> MSKLTQVFKQTKLCIGYLTAGDGGTSYTIEAAKALIQGGVDILELGFPFSDPVADNPEIQVSHDRALAENLTSETLLEIVEGIRAFNQEVPLILYSYYNPLLQRDLDYLRRLKDAGINGVCVIDLPAPLSHGEKSPFFEDLLAVGLDPILLISAGTTPERMSLIQEYARGFLYYIPCQATRDSEVGIKEEFRKVREHFDLPIVDRRDI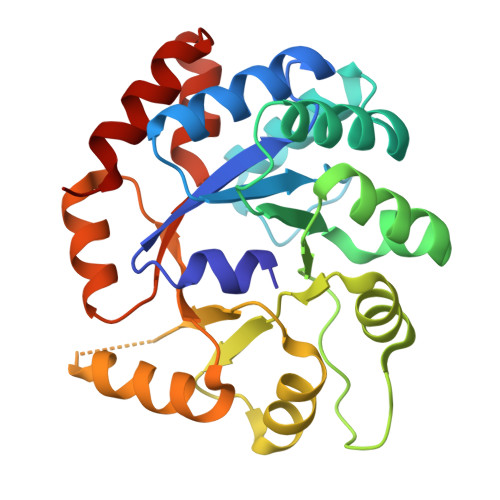CDKKEAAHVLNYSDGFIVKTAFVHQTTMDSSVETLTALAQTVIPG> MAIAFEHVTYTYQAGTPMAHTALTDVSLTVPDRGYLAIIGHTGSGKSTLIQQLNALLKPTSGTIKIDEFTITPETTNAALKPLRQHVGMVFQFPENQLFEETVRQDIAFGPKNFGMADADALALADEMLTTVGLDQSYAERSPFELSGGQMRRVAIAGVLAMQPKVLVLDEPTAGLDPQGRQEMMRLFARLHQEQGLTIVLVTHQMEDVAQYAEQVAVMHEGRLMK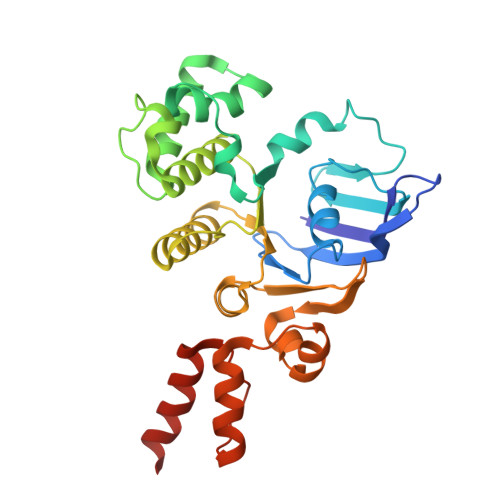FGTPADVFSNREWLQDHQLDVPQAAQFARRLRDRGLTFPKQPLTADQLADYLAQQWAQRGADHV BgaA is specific for galactose β-1,4-linked to glucose or GlcNAc [lactose or N-acetyllactosamine (LacNAc) motifs, respectively] found in glycoconjugates. The N-terminal region of BgaA comprising amino acid residues 138–993 has amino acid sequence identity with GH family 2 enzymes. Through detailed structural and functional analyses the molecular basis for the catalytic specificity of BgaA is defined and this activity is demonstrated as critical for the ability of pneumococci to utilize complex N-linked glycans as a carbon source and protect the bacterium from opsonophagocytic killing. Further analyses also revealed the presence of non-catalytic CBMs within the C-terminal region of BgaA that mediate adherence to host cell surface LacNAc and/or lactose.

The X-ray crystal structures of a catalytically active fragment of BgaA was determined to 2.7 Å resolution (data not shown) and an inactive Glu645Gln nucleophile mutant in complex with unhydrolyzed LacNAc to 2.2 Å resolution. This polypeptide had five distinct domains, four with immunoglobulin (Ig)-like folds that are arranged to create a nest in which the central (α/β)8-barrel domain III sits. The positions of the nucleophile and catalytic acid, Glu645 and Glu564, respectively, in BgaA are conserved with the analogous residues Glu537 and Glu461 of LacZ. Notably, however, there was no evidence of bound metals in the active site of BgaA. Indeed, the side chain of Arg288 occupies the space where a Mg2+ atom is bound in LacZ while Tyr713 and Glu716 fill the region occupied by a Na+ atom. Consistent with this, the activity of our catalytic region construct displayed no sensitivity to the presence or absence of metal ions (data not shown).

> AVTNEEVNQMIEDRKVDFNQNWYFKLNANSKEAIKPDADVSTWKKLDLPYDWSIFNDFDHESPAQNEGGQLNGGEAWYRKTFKLDEKDLKKNVRLTFDGVYMDSQVYVNGQLVGHYPNGYNQFSYDITKYLQKDGRENVIAVHAVNKQPSSRWYSGSGIYRDVTLQVTDKVHVEKNGTTILTPKLEEQQHGKVETHVTSKIVNTDDKDHELVAEYQIVERGGHAVTGLVRTASRTLKAHESTSLDAILEVERPKLWTVLNDKPALYELITRVYRDGQLVDAKKDLFGYRYYHWTPNEGFSLNGERIKFHGVSLHHDHGALGAEENYKAEYRRLKQMKEMGVNSIRTTHNPASEQTLQIAAELGLLVQEEAFDTWYGGKKPYDYGRFFEKDATHPEARKGEKWSDFDLRTMVERGKNNPAIFMWSIGNEIGEANGDAHSLATVKRLVKVIKDVDKTRYVTMGADKFRFGNGSGGHEKIADELDAVGFNYSEDNYKALRAKHPKWLIYGSETSSATRTRGSYYRPERELKHSNGPERNYEQSDYGNDRVGWGKTATASWTFDRDNAGYAGQFIWTGTDYIGEPTPWHNQNQTPVKSSYFGIVDTAGIPKHDFYLYQSQWVSVKKKPMVHLLPHWNWENKELASKVADSEGKIPVRAYSNASSVELFLNGKSLGLKTFNKKQTSDGRTYQEGANANELYLEWKVAYQPGTLEAIARDESGKEIARDKITTAGKPAAVRLIKEDHAIAADGKDLTYIYYEIVDSQGNVVPTANNLVRFQLHGQGQLVGVDNGEQASRERYKAQADGSWIRKAFNGKGVAIVKSTEQAGKFTLTAHSDLLKSNQVTVFTGKKEG>[2x]MQTEHVILLNAQGVPTGTLEKYAAHTADTRLHLAFSSWLFNAKGQLLVTRRALSKKAWPGVWTNSVAGHPQLGESNEDAVIRRCR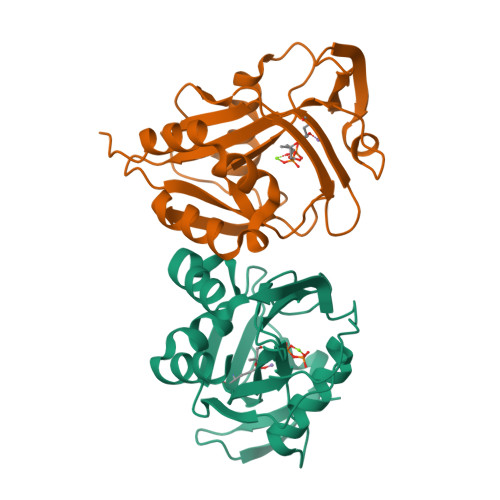YELGVEITPPESIYPDFRYRATDPSGIVENEVCPVFAARTTSALQINDDEVMDYQWCDLADVLHGIDATPWAFSPWMVMQATNREARKRLSAFTQLKL3-tert-butyl-N-[(1S)-6-{2-[5-methyl-1-(propan-2-yl)-1H-pyrazol-4-yl]-1H-imidazo[4,5-b]pyridin-7-yl}-1,2,3,4-tetrahydronaphthalen-1-yl]-1,2,4-oxadiazole-5-carboxamide 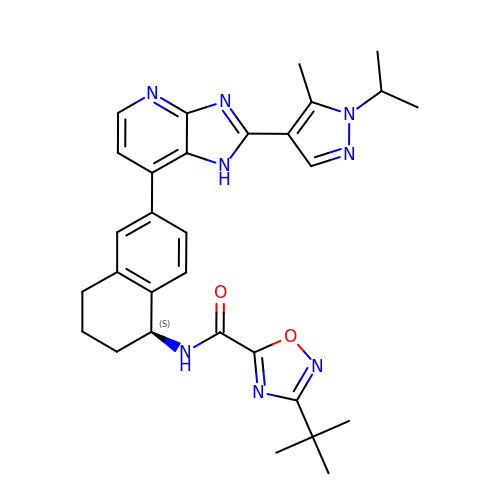| C30 H34 N8 O2 | YHVGIUIWPVYQHA-QHCPKHFHSA-N>MALAKRIDAALILKDGRVVKGSNFENLRDSGDPVELGKFYSEIGIDELSFWDITASVEKRKTMLELVEKVAEQIDIPITVGGGIYDFETASELILRGADKVEINTAAVENPSLITQIAQTFGSQAVVVYIAAKRVDGEFMVFTYSGTKNTGILLRDWVVEVEKRGAGEIVLGSIDRLGTKSG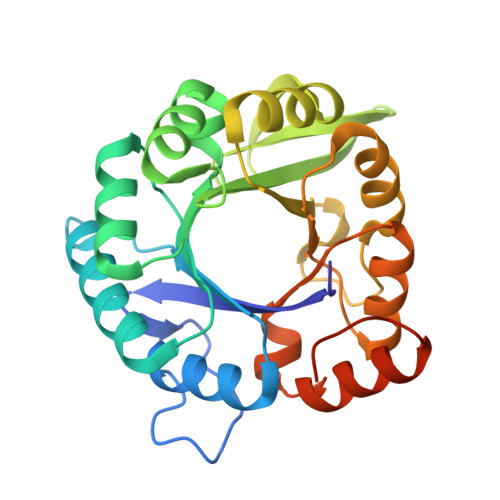YDTEMIRFVRPLTTLPIIAHRGAGKTEHFLEAFLAGADAAKADSVFHSREIDVRELKEYLKKHGVNVRLEGLGSLEHHHHHH[2x]>[2x]MKQYLELMQKVLDEGTQKNDRTGTGTLSIFGHQMRFNLQDGFPLVTTKRCHLRSIIHELLWFLQGDTNIAYLHENNVTIWDEWADENGDLGPVYGKQWRAWPTPDGRHIDQITTVLNQLKNDPD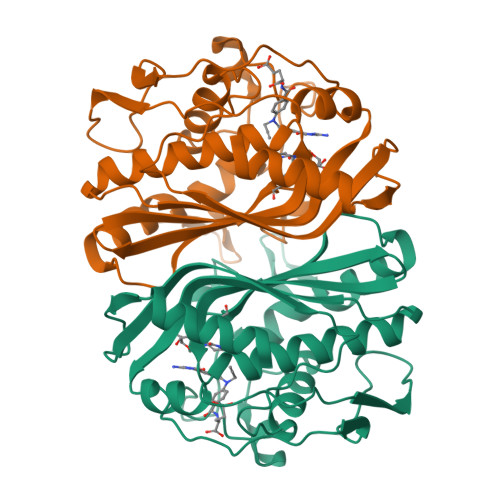SRRIIVSAWNVGELDKMALAPCHAFFQFYVADGKLSCQLYQRSCDVFLGLPFNIASYALLVHMMAQQCDLEVGDFVWTGGDTHLYSNHMDQTHLQLSREPRPLPKLIIKRAPESIFDYRFEDFEIEGYDPHPGIKAPVAI>[2x]MAHHHHHHQKLVEDALNECYNANASDPVGFLGHFFLNRGKKGAVNRVDKLVGREILDSRGNPTVEVDVYANGQKRPVATASAPSGASTGSNEAHELRDGDKSRYLGKGVLKAVKNVNDVLGKAVEGKSLENLTELDQALIDADGDELKSNLGGNAITACSFALATAGAAVRNEELFLYLARAFHGADKFENLKFRLPTPMVNILNGGKHAGGRLQIQEFMILPKENQPFREKVRCVAEVY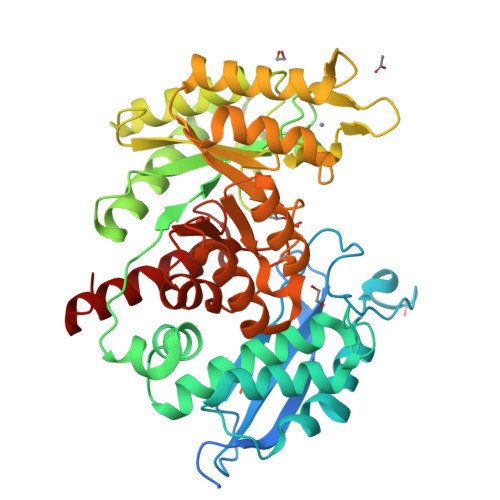QHLGKILAERAGPSAKNVGDEGGFAPNLETADEALNYIEEAIGKAGYKVGEDVFLALDAASSEFYNSDTKKYEITQQKEFLTSEEMVEYYVQLVNRHPAIISIEDGLEEKDYEGWKLLTERLGSKIMLVGDDLYTTNTRLIKQGIEEKWANALLLKVNQIGTITEAMNAARMIFNVGQKVIVSHRSGETATTLISDLVVGIGATHIKTGATARGERVSKYNRLLQIEEYLEQHGLLA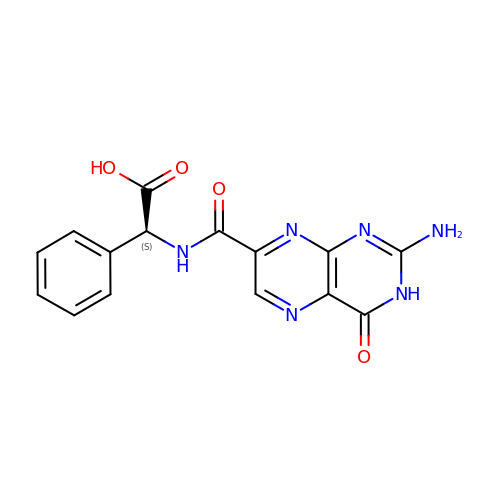(2S)-2-[(2-azanyl-4-oxidanylidene-3H-pteridin-7-yl)carbonylamino]-2-phenyl-ethanoic acid | C15 H12 N6 O4 | CKTFFRDVMHUKQB-VIFPVBQESA-N Expanding this pattern to hpphhph can produce larger α-helical barrels. Here, we show that pentameric to nonameric barrels are accessed by varying the residue at one of the h sites. In peptides with four L/I–K–E–I–A–x–Z repeats, decreasing the size of Z from threonine to serine to alanine to glycine gives progressively larger oligomers. X-ray crystal structures of the resulting α-helical barrels rationalize this: side chains at Z point directly into the helical interfaces, and smaller residues allow closer helix contacts and larger assemblies.

Conversely, both Gly variants scored more favourably as larger oligomeric states: the a = d = Ile variant as an octamer; and a = Leu, d = Ile as a nonamer. The Gly@g variant with a = d = Ile unfolded at 38 °C and did not fully refold on cooling. Indeed, peptide sequences with a = d = Ile are more unstable than their a = Leu, d = Ile counterparts. Thus, β-branched Ile at both a and d maintains the open assembly even with Gly residues at g. Although a larger oligomer was predicted in silico, the calculated internal energies for Gly@g were similar for the different oligomers (Fig. S1†). The hexameric and heptameric assemblies of CC-Type2-(GgIaId)4 imply that, whilst Gly@g is necessary to access larger states, it is not the only factor that dictates oligomer state of the helical assembly.

>[3x]XGEIAQGIKEIAKGIKEIAWGIKEIAQGIKGX>MGHHHHHHMSSQTERTFIAVKPDGVQRGLVSQILSRFEKKGYKLVAIKLVKADDKLLEQHYAEHVGKPFFPKMVSFMKSGPILATVWEGKDVVRQGRTILGATNPLGSAPGTIRGDFGIDLGRNVCHGSDSVDSAEREINLWFKKEE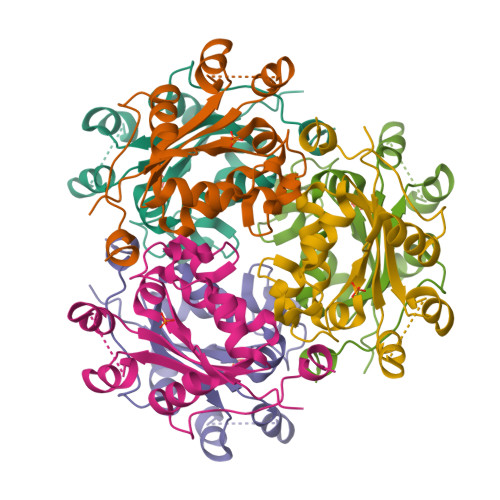LVDWESNQAKWIYE[2x]>[6x]GLRQAVMLPEGEDLNEWIAVNTVDFFNQINMLYGTITEFCTEASCPVMSAGPRYEYHWADGTNIKKPIKCSAPKYIDYLMTWVQDQ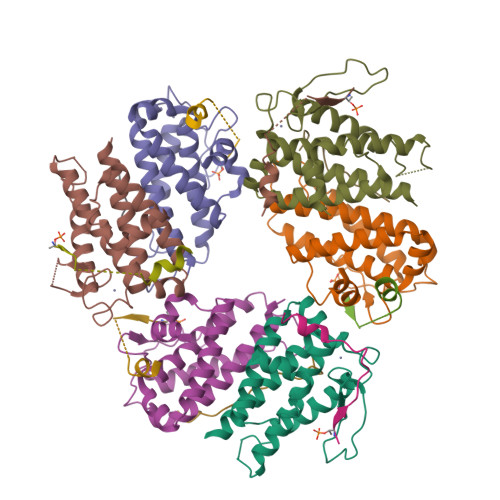LDDETLFPSKIGVPFPKNFMSVAKTILKRLFRVYAHIYHQHFDSVMQLQEEAHLNTSFKHFIFFVQEFNLIDRRELAPLQELIEKLGSKDR;>DEEEEDGTMKRNATSPQVQRPSFMDYFDKQD[9x]> MSVNYAAGLSPYADKGKCGLPEIFDPPEELERKVWELARLVWQSSSVVFHTGAGISTASGIPDFRGPHGVWTMEERGLAPKFDTTFESARPTQTHMALVQLERVGLLRFLVSQNVDGLH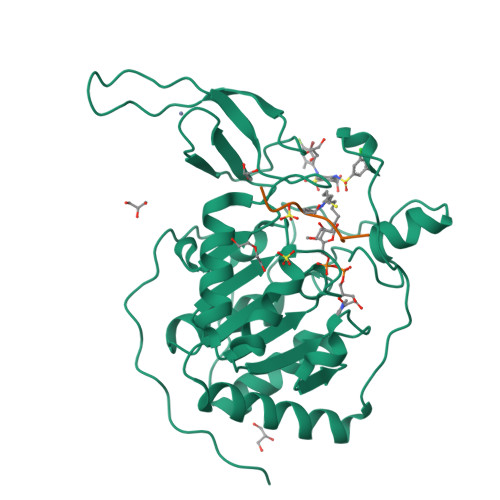VRSGFPRDKLAELHGNMFVEECAKCKTQYVRDTVVGTMGLKATGRLCTVAKARGLRACRGELRDTILDWEDSLPDRDLALADEASRNADLSITLGTSLQIRPSGNLPLATKRRGGRLVIVNLQPTKHDRHADLRIHGYVDEVMTRLMKHLGLEIPAWDGPRVLERALPPLPRPPTPKLEPKEESPTRINGSIPAGPKQEPCAQHNGSEPASPKRERPTSPAPHRPPKRVKAKAVPS;> QTARKSTGG>MKVLVINAGSSSLKYQLIDMTNESALAVGLCERIGIDNSIITQKKFDGKKLEKLTDLPTHKDALEEVVKALTDDEFGVIKDMGEINAVGHRVVHGGEKFTTSALYDEGVEKAIKDCFELAPLHNPPNMMGISACAEIMPGTPMVIVFDTAFHQTMPPYAYMYALPYDLYEKHGVRKYGFHGTSHKYVAERAALMLGKPAEETKIITCHLGNGSSITAVEGGKSVETSMGFTPLEGLAMGTRCGSIDPAIVPFLMEKEGLTTREIDTL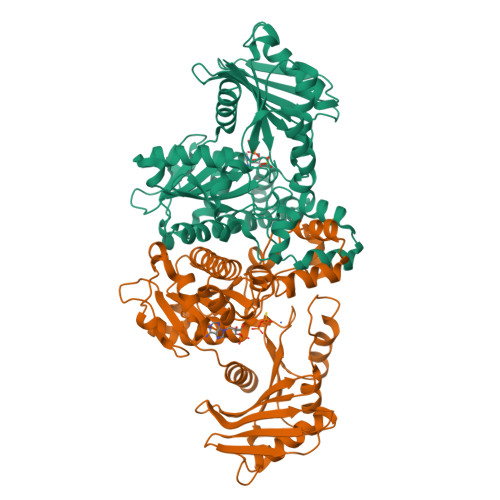MNKKSGVLGVSGLSNDFRDLDEAASKGNRKAELALEIFAYKVKKFIGEYSAVLNGADAVVFTAGIGENSASIRKRILTGLDGIGIKIDDEKNKIRGQEIDISTPDAKVRVFVIPTNEELAIARETKEIVETE[2x]>G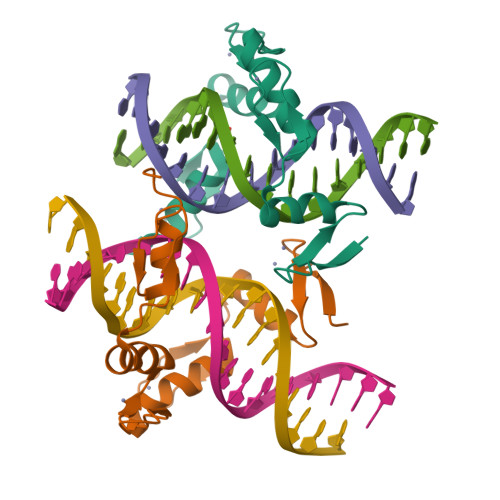SHMQKCPICEKVIQGAGKLPRHIRTHTGEKPYECNICKVRFTRQDKLKVHMRKHTGEKPYLCQQCGAAFAHNYDLKNHMRVHTGLRPYQCDSCCKTFVRSDHLHRHLKKDGCNGVPSRRGRKPRVRGGW[2x]>MPAEYRYKIVMLGDGAVGKTAMTTRFTQNFFDTDYKRTIGSDFAVKRLQLDDINAHVTLQIWDLAGQPRFESVRQGFYRGARGGLLLYDVTRRRTFINIENWKEEAFRSLQKEIPLVVVANKVDLKDSRVVA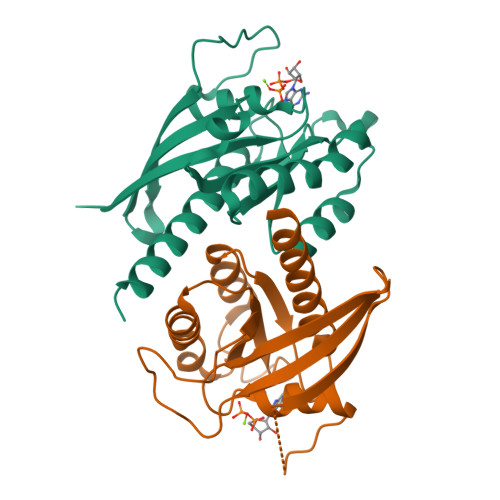TEEGEEYAKNNSFMYVESSALTGENVEEAYANLCRIMIEESKDISEMTST[2x]> QDLTVKMTDLQTGKPVGTIELSQ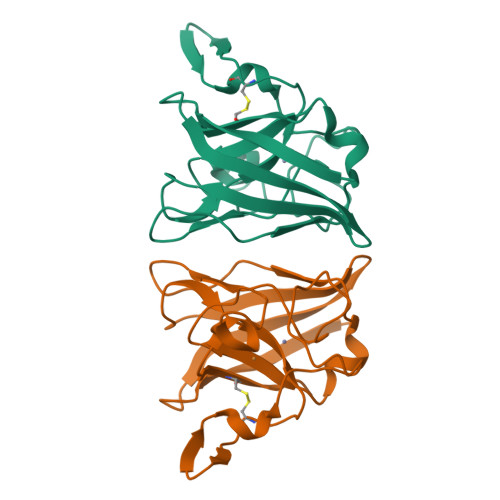NKYGVVFIPELADLTPGMHGFHIHQNGSCASSEKDGKVVLGGAAGGHYDPEHTNKHGFPFTDDNHKGDLPALFVSANGLATNPVLAPRLTLKELKGHAIMIHAGGDNHSDMPKALGGGGARVACGVIQ> EPGDGAQTWARFSRPPAPEAAGLFQGTFPDGFLWAVGSAAYQTEGGWQQHGKGASIWDTFTHHPLAPPGDSRNASLPLGAPSPLQPATGDVASDSYNNVFRDTEALRELGVTHYRFSISWARVLPNGSAGVPNREGLRYYRRLLERLRELGVQPVVTLYHWDLPQRLQDAYGGWANRALADHFRDYAELCFRHFGGQVKYWITIDNPYVVAWHGYATGRLAPGIRGSPRLGYLVAHNLLLAHAKVWHLYNTSFRPTQGGQVSIALSSHWINPRRMTDHSIKECQKSLDFVLGWFAKPVFIDGDYPESMKNNLSSILPDFTESEKKFIKGTADFFALCFGPTLSFQLLDPHMKFRQLESPNLRQLLSWIDLEFNHPQIFIVENGWFVSGTTKRDDAKYMYYLKKFIMETLKAIKLDGVDVIGYTAWSLMDGFEWHRGYSIRRGLFYVDFLSQDKMLLPKSSALFYQKLIEKNGFPPLPENQPLEGTFPCDFAWGVVDNYIQVDTTLSQFTDLNVYLWDVHHSKRLIKVDGVVTKKRKSYCVDFAAIQPQIALLQEMHVTHFRFSLDWALILPLGNQSQVNHTILQYYRCMASELVRVNITPVVALWQPMAPNQGLPRLLARQGAWENPYTALAFAEYARLCFQELGHHVKLWITMNEPYTRNMTYSAGHNLLKAHALAWHVYNEKFRHAQNGKISIALQADWIEPACPFSQKDKEVAERVLEFDIGWLAEPIFGSGDYPWVMRDWLNQRNNFLLPYFTEDEKKLIQGTFDFLALSHYTTILVDSEKEDPIKYNDYLEVQEMTDITWLNSPSQVAVVPWGLRKVLNWLKFKYGDLPMYIISNGIDDGLHAEDDQLRVYYMQNYINEALKAHILDGINLCGYFAYSFNDRTAPRFGLYRYAADQFEPKASMKHYRKIIDSNGFPGPETLERFCPEEFTVCTECSF;> YPNASPLLGSSWGGLIHLYTATARNSYHLQIHKNGHVDGAPHQTIYSALMIRSEDAGFVVITGVMSRRYLCMDFRGNIFGSHYFDPENCRFQHQTLENGYDVYHSPQYHFLVSLGRAKRAFLPGMNPPPYSQFLSRRNEIPLIHFNTPIPRQHTQSAEDDSERDPLNVLKPRARMTPAP;>YPQQAPYWTHPQRMEKKLHAVPAGNTVKFRCPAAGNPTPTIRWLKDGQAFHGENRIGGIRLRHQHWSLVMESVVPSDRGTYTCLVENAVGSIRYNYLLDVLERSPHRPILQAGLPANTTAVVGSDVELLCKVYSDAQPHIQWLKHIVINGSSFGADGFPYVQVLKTADINSSEVEVLYLRNVSAEDAGEYTCLAGNSIGLSYQSAWLTVLPEE[2x]

To reveal the molecular mechanism underpinning the coreceptor role of HS, we solved cryo-electron microscopy structures of three distinct 1:2:1:1 FGF23–FGFR–αKlotho–HS quaternary complexes featuring the ‘c’ splice isoforms of FGFR1 (FGFR1c), FGFR3 (FGFR3c) or FGFR4 as the receptor component. Contrary to our prediction, all three cryo-EM structures reveal identical asymmetric 1:2:1:1 FGF23–FGFR–αKlotho–HS quaternary assemblies in which HS enables a 1:1:1 FGF23–FGFR–αKlotho ternary complex to recruit a lone FGFR chain (termed FGFRS to differentiate it from the ‘primary’ receptor FGFRP within the ternary complex). At the membrane distal end of each quaternary complex, HS engages in tripartite interactions with juxtaposed HS binding sites of FGF23, FGFRP and FGFRS. In doing so, HS augments interactions of FGF23 and FGFRP from the FGF23–FGFRP–αKlotho ternary complex with the FGFRS chain, and thus induces receptor (that is, FGFRP–FGFRS) dimerization.

The direct FGFRP–FGFRS contacts bury a modest solvent-exposed surface area (1542.6 Å2) and are preserved among the three cryo-EM structures. Akin to the FGFRP–FGFRS interface, the FGF23–FGFRS interface is also conserved among the three quaternary complexes and masks a rather modest surface exposed area (1668.6 Å2). We targeted site 2 of the FGFRP–FGFRS interface in each of the three quaternary complexes by introducing four different point mutations individually into full-length FGFR1c (E249A, R254A, I256A, Y280A), FGFR3c (E247A, R252A, I254A, Y278A) or FGFR4 (E243A, R248A, I250A, Y274A). As in the case of the L6-FGFR1cWT cell line, cotreatment with FGF23 and soluble αKlotho of L6-FGFR3cWT and L6-FGFR4WT cell lines robustly stimulated FGFR signalling as detected by phosphorylation/activation of FGFRs and downstream PLCγ1/FRS2α/ERK signal transducers. In contrast, cells expressing mutated FGFR1c, FGFR3c and FGFR4 had diminished FGFR A-loop tyrosine phosphorylation and reduced PLCγ1, FRS2α and MAPK activation. Specifically, we reasoned that a primary FGFR1cP should be able to pair with FGFR3c or FGFR4 as the secondary receptor to yield functional 1:2:1:1 FGF23–FGFR1c–FGFR3c–αKlotho–HS or FGF23–FGFR1c–FGFR4–αKloth–HS heterodimeric quaternary complexes. To test this possibility, we carried out a receptor complementation assay using an FGFR4 variant harbouring a double I197E/S217E mutation (termed FGFR4ΔSLBS)—corresponding to FGFR1cΔSLBS—as the primary receptor and FGFR1cΔPLBS as the secondary receptor. However, robust activation of an FGFR signalling pathway took place in the L6-FGFR1cΔPLBS + FGFR4ΔSLBS co-expressing cell line. In contrast, copious and intense punctate fluorescent spots appeared on the surface of L6-FGFR1cΔPLBS + FGFR4ΔSLBS co-expressing cells, which implies that an FGF23–FGFR1c–FGFR4–αKlotho–HS heterodimeric quaternary complex can form on the surface of live cells.>EDPHLRNRPGKGHNYIDGMTQEDATCKPVTYAGACSSFDVLLEKGKFPLFQSYAHHRTLLEAVHDTIIAKADPPSCDLQSAHGNPCMKEKLVMKTHCPNDYQSAHYLNNDGKMASVKCPPKYELTEDCNFCRQMTGASLKKGSYPLQDLFCQSSEDDGSKLKTKMKGVCEVGVQALKKCDGQLSTAHEVVPFAVFKNSKKVYLDKLDLKTEENLLPDSFVCFEHKGQYKGKLDSGQTKRELKSFDISQCPKIGGHGSKKCTGDAAFCSAYECTAQYANAYCSHANGSGIVQIQVSGVWKKPLCVGYERVVVKRELS[6x];>DPGCSELIQASSRITTCSTEGVNTKCRLSGTALIRAGSVGAEACLMLKGVKEDQTKFLKIKTVSSELSCREGQSYWTGSFSPKCLSSRRCHLVGECHVNRCLSWRDNETSAEFSFVGESTTMRENKCFEQCGGWGCGCFNVNPSCLFVHTYLQSVRKEALRVFNCIDWVHKLTLEITDFDGSVSTIDLGASSSRFTNWGSVSLSLDAEGISGSNSFSFIESPGKGYAIVDEPFSEIPRQGFLGEIRCNSESSVLSAHESCLRAPNLISYKPMIDQLECTTNLIDPFVVFERGSLPQTRNDKTFAASKGNRGVQAFSKGSVQADLTLMFDNFEVDFVGAAVSCDAAFLNLTGCYSCNAGARVCLSITSTGTGSLSAHNKDGSLHIVLPSENGTKDQCQILHFTVP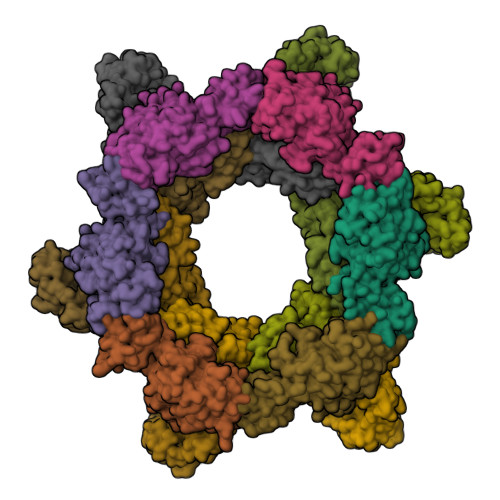EVEEEFMYSCDGDERPLLVKGTLIAID[6x]4-[(4,4-DIMETHYL-1,2,3,4-TETRAHYDRO-[1,2']BINAPTHALENYL-7-CARBONYL)-AMINO]-BENZOIC 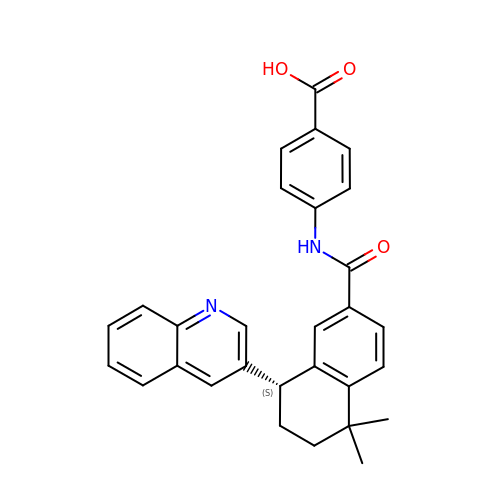ACID | C29 H26 N2 O3 | WBEIHCAWTAWTBK-UHFFFAOYSA-N> GT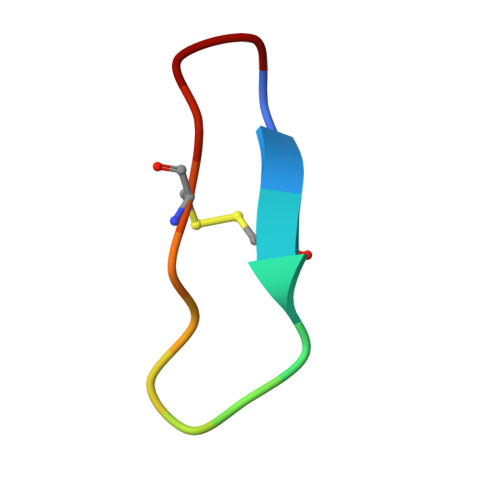CTRSIPPICNPN>[2x]MSKIRIGIVGYGNLGRGVEAAIQQNPDMELVAVFTRRDPKTVAVKSNVKVLHVDDAQSYKDEIDVMILCGGSATDLPEQGPYFAQYFNTIDSFDTHARIPDYFDAVNAAAEQSGKVAIISVGWDPGLFSLNRLLGEVVLPVGNTYTFWGKGVSQGHSDAIRRIQGVKNAV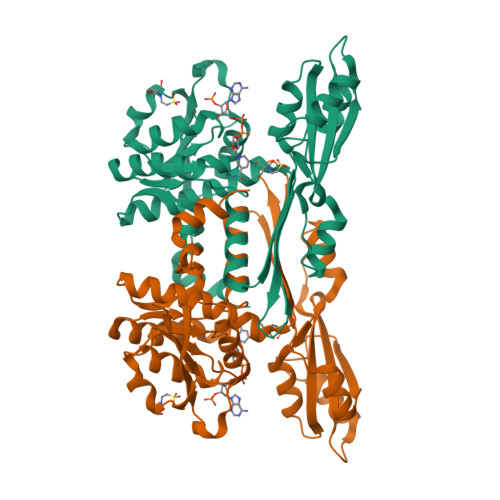QYTIPIDEAVNRVRSGENPELSTREKHARECFVVLEEGADPAKVEHEIKTMPNYFDEYDTTVHFISEEELKQNHSGMPHGGFVIRSGKSDEGHKQIIEFSLNLESNPMFTSSALVAYARAAYRLSQNGDKGAKTVFDIPFGLLSPKSPEDLRKELLTRHHHHHH>[2x]KMAFTLADRVTEEMLADKAALVVEVVEENYHDAPIVGIAVVNEHGRFFLRPETALADPQFVAWLGDETKKKSMFDSKRAAVALKWKGIELCGVSFDLLLAAYLLDPAQGVDDVAAAAKMKQYEAVRPDEAVYGKGAKRAVPDEPVLAEHLVRKAAAIWELERPFLDELRRNEQDRLLVELEQPLSSILAEMEFAGVKVDTKRLEQMGKELAEQLGTVEQRIYELAGQEFNINSPKQLGVILFEKLQLPVLKKTKTGYSTSADVLEKLAPYHEIVENILHYRQLGKLQSTYIEGLLKVVRPATKKVHTIFNQALTQTGRLSSTEPNLQNIPIRLEEGRKIRQAFVPSESDWLIFAADYSQIELRVLAHIAEDDNLMEAFRRDLDIH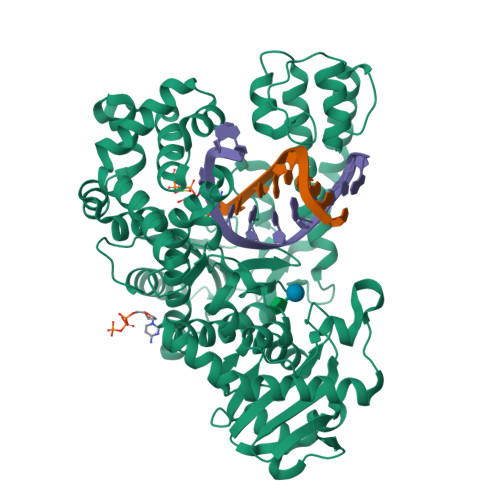TKTAMDIFQVSEDEVTPNMRRQAKAVNFGIPYGISDYGLAQNLNISRKEAAEFIERYFESFPGVKRYMENIVQEAKQKGYVTTLLHRRRYLPDITSRNFNVRSFAERMAMNTPIQGSAADIIKKAMIDLNARLKEERLQAHLLLQVHDELILEAPKEEMERLCRLVPEVMEQAVTLRVPLKVDYHYGSTWYDAK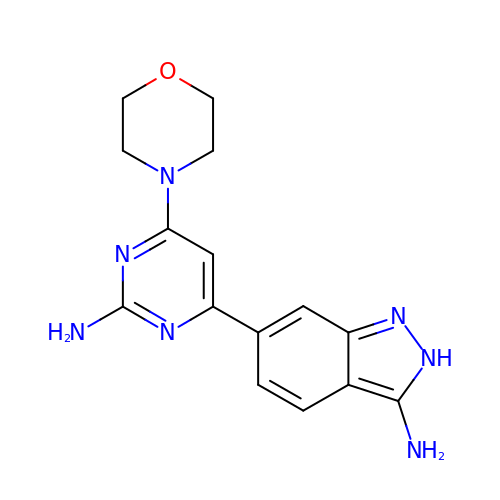6-[2-amino-6-(morpholin-4-yl)pyrimidin-4-yl]-2H-indazol-3-amine | C15 H17 N7 O | IBSXLFOFZRSWEZ-UHFFFAOYSA-N>[2x]MATDLKASSLRALKLMHLATSANDDDTDENVIALCHQAKTPVGNTDAIFIYPRFIPIARKTLKEQGTPEIRICTSTNFPHGNDDIDIALAETRAAIAYGADSVAVVFPYRALMAGNEQVGFDLVKACKEACAAANVLLAVIIETGELKDEALIRKASEISIKAGADNI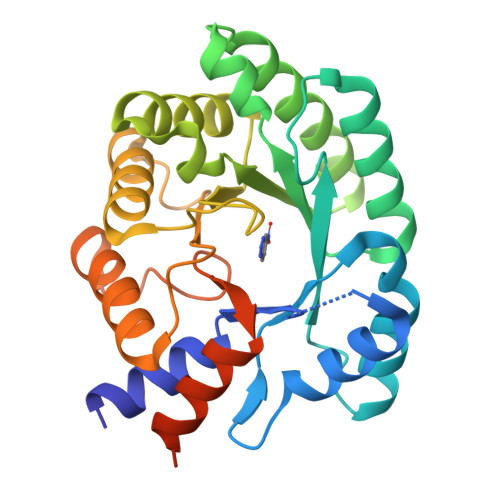VTSTGKVAVGATPESARIMMEVIRDMGVEKTVGFIPVGGVRTAEDAQKYLAIADELFGADWADARHYAFGASASLLASLLKALGHGDGKSASSYGSLEHHHHHH>MASNQEEVKVYGMMASPFVSRVEIALKLKGVEYKYELEKFGNFSDTLIKYNPVYKKVPVFVHNDRPISESLVILEYIDETWKQNPLLPSDPYKRALVRFWTKFIDDKCLSAARKATFSIDEKEREKGIEETEEAFQILENELKDKFFGGDEIGIVDIAGIFIAFWFPIVQEATRLKLFTSEKFPKLHKWSED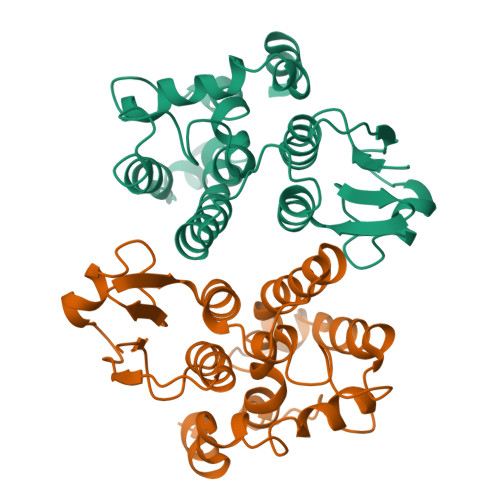LSNHPIVKEILPPRESLLAYFKARYESLTASK[2x]> PSSEQAWLEDAQVFIQKTLCPAVKEPNVQLTPLVIDCVKTVWLSQGRNQGSTLPLSYSFVSVQDLKTHQRLPCCSHLSWSSSAYQAWAQEAGPNGNPLPREQLLLLGTLTDLSADLEQECRNGSLYVRDNTGVLSCELIDLDLSWLGHLFLFPRWSYLPPARWNSSGEGHLELWDAPVPVFPLTISPGPVTPIPVLYPESASCLLRLRNKLRGVQRNLAGSLVRLSALVKSKQKAYFILSLGRSHPAVTHVSIIVQVPAQLVWHRALRPGTAYVLTELRVSKIRGQRQHVWMTSQSSRLLLLKPECVQELELELEGPLLEADPKPLPMPSNSEDKKDPESLVRYSRLLSYSGAVTGVLNEPAGLYELDGQLGLCLAYQQFRGLRRVMRPGVCLQLQDVHLLQSVGGGTRRPVLAPCLRGAVLLQSFSRQKPGAHSSRQAYGASLYEQLVWERQLGLPLYLWATKALEELACKLCPHVLRHHQFLQHSSPGSPSLGLQLLAPTLDLLAPPGSPVRNAHNEILEEPHHCPLQKYTRLQTPSSFPTLATLKEEGQRKAWASFDPKALLPLPEASYLPSCQLNRRLAWSWLCLLPSAFCPAQVLLGVLVASSHKGCLQLRDQSGSLPCLLLAKHSQPLSDPRLIGCLVRAERFQLIVERDVRSSFPSWKELSMPGFIQKQQARVYVQFFLADALILPVPRPCLHSATPSTPQTDPTGPEGPHLGQSRLFLLCHKEALMKRNFCVPPGASPEVPKPALSFYVLGSWLGGTQRKEGTGWGLPEPQGNDDNDQKVHLIFFGSSVRWFEFLHPGQVYRLVAPGPATPMLFEKDGSSCISRRPLELAGCASCLTVQDNWTLELESSQDIQDVLDANKSLPESSLTDLLSDNFTDSLVSFSAEILSRTLCEPLVASLWMKLGNTGAMRRCVKLTVALETAECEFPPHLDVYIEDPHLPPSLGLLPGARVHFSQLEKRVSRSHNVYCCFRSSTYVQVLSFPPETTISVPLPHIYLAELLQGGQSPFQATASCHIVSVFSLQLFWVCAYCTSICRQGKCTRLGSTCPTQTAISQAIIRLLVEDGTAEAVVTCRNHHVAAALGLCPREWASLLDFVQVPGRVVLQFAGPGAQLESSARVDEPMTMFLWTLCTSPSVLRPIVLSFELERKPSKIVPLEPPRLQRFQCGELPFLTHVNPRLRLSCLSIRESEYSSSLGILASSC;> RCEEETPSLLWGLDPVFLAFAKLYIRDILDMKESRQVPGVFLYNGHPIKQVDVLGTVIGVRERDAFYSYGVDDSTGVINCICWKKLNTESVSAAPSAARELSLTSQLKKLQETIEQKTKIEIGDTIRVRGSIRTYREEREIHATTYYKVDDPVWNIQIARMLELPTIYRKVYDQPFHSSALEKEEALSNPGALDLPSLTSLLSEKAKEFLMENRVQSFYQQELEMVESLLSLANQPVIHSASSDQVNFKKDTTSKAIHSIFKNAIQLLQEKGLVFQKDDGFDNLYYVTREDKDLHRKIHRIIQQDCQKPNHMEKGCHFLHILACARLSIRPGLSEAVLQQVLELLEDQSDIVSTMEHYYTAF;> LPKPGTYYLPWEVSAGQVPDGSTLRTFGRLCLYDMIQSRVTLMAQHGSDQHQVLVCTKLVEPFHAQVGSLYIVLGELQHQQDRGSVVKARVLTCVEGMNLPLLEQAIREQRLYKQERGGSQ;> ETFDPTELPELLKLYYRRLFPYSQYYRWLNYGGVIKNYFQHREFSFTLKDDIYIRYQSFNNQSDLEKEMQKMNPYKIDIGAVYSHRPNQHNTVKLGAFQAQEKELVFDIDMTDYDDVRRCCSSADICPKCWTLMTMAIRIIDRALKEDFGFKHRLWVYSGRRGVHCWVCDESVRKLSSAVRSGIVEYLSLVKGGQDVKKKVHLSEKIHPFIRKSINIIKKYFEEYALVNQDILENKESWDKILALVPETIHDELQQSFQKSHNSLQRWEHLKKVASRYQNNIKNDKYGPWLEWEIMLQYCFPRLDINVSKGINHLLKSPFSVHPKTGRISVPIDLQKVDQFDPFTVPTISFICRELDAISTNEEEKEENEAESDVKHRTRDYKKTSLAPYVKVFEHFLENLDKSRKGELLKKSDLQKDF;> DQRNASYPHCLQFYLQPPSENISLIEFENLAIDRVKLLKSVENLGVSYVKGTEQYQSKLESELRKLKFSYRENLEDEYEPRRRDHISHFILRLAYCQSEELRRWFIQQEMDLLRFRFSILPKDKIQDFLKDSQLQFEAISDEEKTLREQEIVASSPSLSGLKLGFESIYKIPFADALDLFRGRKVYLEDGFAYVPLKDIVAIILNEFRAKLSKALALTARSLPAVQSDERLQPLLNHLSHS;> VDSSHLPLVKGADEEQVFHFYWLDAYEDQYNQPGVVFLFGKVWIESAETHVSCCVMVKNIERTLYFLPREMKIDLNTGKETGTPISMKDVYEEFDEKIATKYKIMKFKSKPVEKNYAFEIPDVPEKSEYLEVKYSAEMPQLPQDLKGETFSHVFGTNTSSLELFLMNRKIKGPCWLEVKSPQLLNQPVSWCKVEAMALKPDLVNVIKDVSPPPLVVMAFSMKTMQNAKNHQNEIIAMAALVHHSFALDKAAPKPPFQSHFCVVSKPKDCIFPYAFKEVIEKKNVKVEVAATERTLLGFFLAKVHKIDPDIIVGHNIYGFELEVLLQRINVCKAPHWSKIGRLKRSNMPKLGGRSGFGERNATCGRMICDVEISAKELIRCKSYHLSELVQQILKTERVVIPMENIQNMYSESSQLLYLLEHTWKDAKFILQIMCELNVLPLALQITNIAGNIMSRTLMGGRSERNEFLLLHAFYENNYIVPDKQIFRKPQQKLGDEDEEIDGDTNKYKKGRKKAAYAGGLVLDPKVGFYDKFILLLDFNSLYPSIIQEFNICFTTVQRVASEAQKVTEDGEQEQIPELPDPSLEMGILPREIRKLVERRKQVKQLMKQQDLNPDLILQYDIRQKALKLTANSMYGCLGFSYSRFYAKPLAALVTYKGREILMHTKEMVQKMNLEVIYGDTDSIMINTNSTNLEEVFKLGNKVKSEVNKLYKLLEIDIDGVFKSLLLLKKKKYAALVVEPTSDGNYVTKQELKGLDIVRRDWCDLAKDTGNFVIGQILSDQSRDTIVENIQKRLIEIGENVLNGSVPVSQFEINKALTKDPQDYPDKKSLPHVHVALWINSQGGRKVKAGDTVSYVICQDGSNLTASQRAYAPEQLQKQDNLTIDTQYYLAQQIHPVVARICEPIDGIDAVLIATWLGLDPTQFRVHHYHKDEENDALLGGPAQLTDEEKYRDCERFKCPCPTCGTENIYDNVFDGSGTDMEPSLYRCSNIDC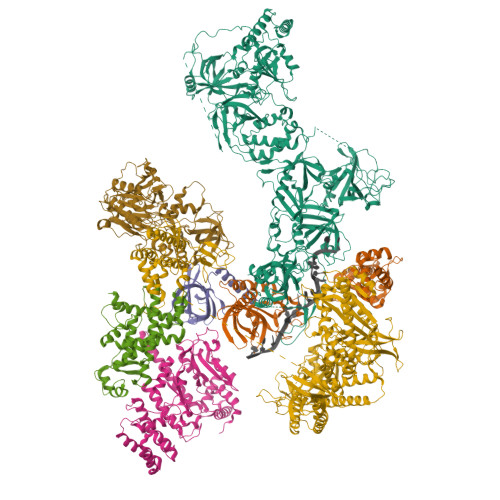KASPLTFTVQLSNKLIMDIRRFIKKYYDGWLICEEPTCRNRTRHLPLQFSRTGPLCPACMKATLQPEYSDKSLYTQLCFYRYIFDAECALEKLTTDHEKDKLKKQFFTPKVLQDYRKLKNTAEQFLSRSGYSEVNLSKLFAGCAVKS;> HQLLSPSSFSPSATPSQKYNSRSNRGEVVTSFGLAQGVSWSGRGGAGNISLKVLGCPEALTGSYKSMFQKLPDIREVLTCKIEELGSELKEHYKIEAFTPLLAPAQEPVTLLGQIGCDSNGKLNNKSVILEGDREHSSGAQIPVDLSELKEYSLFPGQVVIMEGINTTGRKLVATKLYEGVPLPFYQPTEEDADFEQSMVLVACGPYTTSDSITYDPLLDLIAVINHDRPDVCILFGPFLDAKHEQVENCLLTSPFEDIFKQCLRTIIEGTRSSGSHLVFVPSLRDVHHEPVYPQPPFSYSDLSREDKKQVQFVSEPCSLSINGVIFGLTSTDLLFHLGAEEISSSSGTSDRFSRILKHILTQRSYYPLYPPQEDMAIDYESFYVYAQLPVTPDVLIIPSELRYFVKDVLGCVCVNPGRLTKGQVGGTFARLYLRRPAADGAERQSPCIAVQVVRI> MEKFAPEFHGEDANNRATKFLESIKGKFTSPKDPKKKDSIISVNSIDIEVTKESPITSNSTIINPTNETDDTAGNKPNYQRKPLVSFKEDPTPSDNPFSKLYKET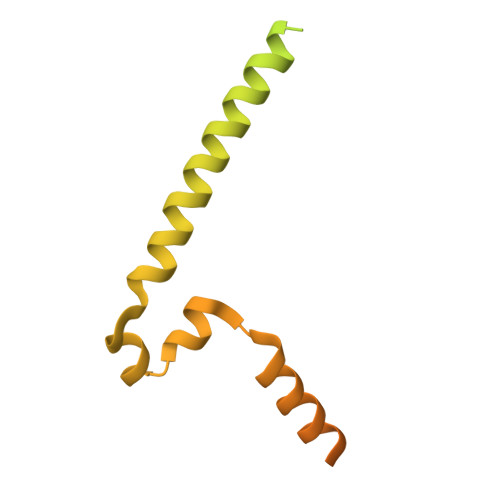IETFDNNEEESSYSYEEINDQTNDNITARLDRIDEKLSEILGMLHTLVVASAGPTSARDGIRDAMVGLREEMIEKIRTEALMTNDRLEAMARLRNEESEKMAKDTSDEVSLNPTSEKLNNLLEGNDSDNDLSLEDF> GSHMASMREFIFKANKTITSSDINLKDL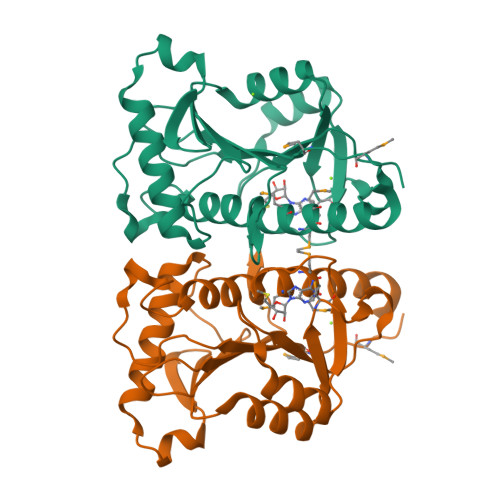PGSCGRLDLLCRCVSDAFFLSHDIRRDVVFYAVLYGQPNPPVCIKFVGSELKKVSPDERNIAIFIKKALKKFEELDEEQRKDWNQSTPGIYVRRLGFRNLVLEKLEEGKNIYYLHMNGEDVENVDIENPVFIIGDHIGIGEEDERFLDEIKAKRISLSPLELHANHCMTMMHNVLDKKRICEI> MLDPGEVYDDPIDPIELEAEPRGTPIVPNILRNSDYNLNSPLIEDPARLMLEWLKTGNRPYRMTLTDNCSRSFRVLKDYFKKVDLGSLKVGGMAAQSMISLWLYGAHSESNRSRRCITDLAHFYSKSSPIEKLLNLTLGNRGLRIPPEGVLSCLERVDYDNAFGRYLANTYSSYLFFHVITLYMNALDWDEEKTILALWKDLTSVDIGKDLVKFKDQIWGLLIVTKDFVYSQSSNCLFDRNYTLMLKDLFLSRFNSLMVLLSPPEPRYSDDLISQLCQLYIAGDQVLSMCGNSGYEVIKILEPYVVNSLVQRAEKFRPLIHSLGDFPVFIKDKVSQLEETFGPCARRFFRAL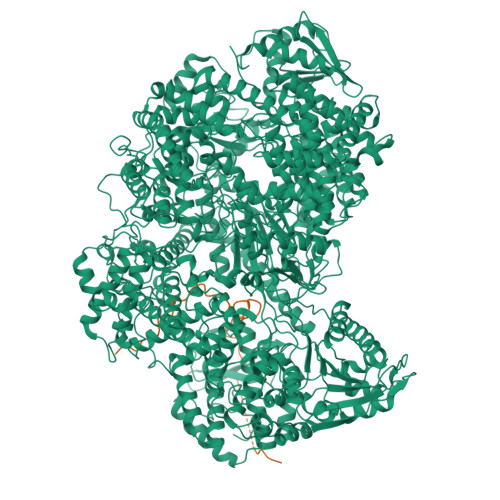DQFDNIHDLVFVFGCYRHWGHPYIDYRKGLSKLYDQVHLKKMIDKSYQECLASDLARRILRWGFDKYSKWYLDSRFLARDHPLTPYIKTQTWPPKHIVDLVGDTWHKLPITQIFEIPESMDPSEILDDKSHSFTRTRLASWLSENRGGPVPSEKVIITALSKPPVNPREFLRSIDLGGLPDEDLIIGLKPKERELKIEGRFFALMSWNLRLYFVITEKLLANYILPLFDALTMTDNLNKVFKKLIDRVTGQGLLDYSRVTYAFHLDYEKWNNHQRLESTEDVFSVLDQVFGLKRVFSRTHEFFQKAWIYYSDRSDLIGLREDQIYCLDASNGPTCWNGQDGGLEGLRQKGWSLVSLLMIDRESQIRNTRTKILAQGDNQVLCPTYMLSPGLSQEGLLYELERISRNALSIYRAVEEGASKLGLIIKKEETMCSYDFLIYGKTPLFRGNILVPESKRWARVSCVSNDQIVNLANIMSTVSTNALTVAQHSQSLIKPMRDFLLMSVQAVFHYLLFSPILKGRVYKILSAEGESFLLAMSRIIYLDPSLGGISGMSLGRFHIRQFSDPVSEGLSFWREIWLSSQESWIHALCQEAGNPDLGERTLESFTRLLEDPTTLNIRGGASPTILLKDAIRKALYDEVDKVENSEFREAILLSKTHRDNFILFLISVEPLFPRFLSELFSSSFLGIPESIIGLIQNSRTIRRQFRKSLSKTLEESFYNSEIHGISRMTQTPQRVGGVWPCSSERADLLREISWGRKVVGTTVPHPSEMLGLLPKSSISCTCGATGGGNPRVSVSVLPSFDQSFFSRGPLKGYLGSSTSMSTQLFHAWEKVTNVHVVKRALSLKESINWFITRDSNLAQALIRNIMSLTGPDFPLEEAPVFKRTGSALHRFKSARYSEGGYSSVCPNLLSHISVSTDTMSDLTQDGKNYDFMFQPLMLYAQTWTSELVQRDTRLRDSTFHWHLRCNRCVRPIDDVTLETSQIFEFPDVSKRISRMVSGAVPHFQRLPDIRLRPGDFESLSGREKSHHIGSAQGLLYSILVAIHDSGYNDGTIFPVNIYGKVSPRDYLRGLARGVLIGSSICFLTRMTNININRPLELVSGVISYILLRLDNHPSLYIMLREPSLRGEIFSIPQKIPAAYPTTMKEGNRSILCYLQHVLRYEREIITASPENDWLWIFSDFRSAKMTYLSLITYQSHLLLQRVERNLSKSMRDNLRQLSSLMRQVLGGHGEDTLESDDNIQRLLKDSLRRTRWVDQEVRHAARTMTGDYSPNKKVSRKVGCSEWVCSAQQVAVSTSANPAPVSELDIRALSKRFQNPLISGLRVVQWATGAHYKLKPILDDLNVFPSLCLVVGDGSGGISRAVLNMFPDAKLVFNSLLEVNDLMASGTHPLPPSAIMRGGNDIVSRVIDLDSIWEKPSDLRNLATWKYFQSVQKQVNMSYDLIICDAEVTDIASINRITLLMSDFALSIDGPLYLVFKTYGTMLVNPNYKAIQHLSRAFPSVTGFITQVTSSFSSELYLRFSKRGKFFRDAEYLTSSTLREMSLVLFNCSSPKSEMQRARSLNYQDLVRGFPEEIISNPYNEMIITLIDSDVESFLVHKMVDDLELQRGTLSKVAIIIAIMIVFSNRVFNVSKPLTDPSFYPPSDPKILRHFNICCSTMMYLSTALGDVPSFARLHDLYNRPITYYFRKQVIRGNVYLSWSWSNDTSVFKRVACNSSLSLSSHWIRLIYKIVKTTRLVGSIKDLSREVERHLHRYNRWITLEDIRSRSSLLDYSCL;> XXXXXEDMGRLHLDDGKSPNHGEIAKVGEGKYREDFQMDEGE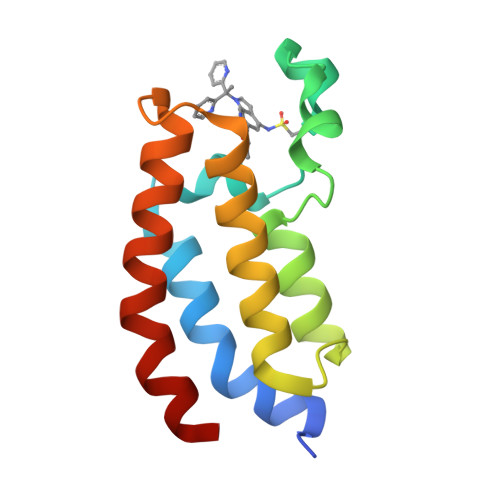>[8x]GSKKIFKPEELRQALMPTLEALYRQDPESLPFRQPVDPQLLGIPDYFDIVKNPMDLSTIKRKLDTGQYQEPWQYVDDVWLMFNNAWLYNRKTSRVYKFCSKLAEVFEQEIDPVMQSLG> MGSSHHHHHHSQDPNSMTTLTRQDLNFGQVVADVLCEFLEVAVHLILYVREVYPVGIFQKRKKYNVPVQMSCHPELNQYIQDTLHCVKPLLEKNDVEKVVVVILDKEHRPVEKFVFEITQPPLLSISSDSLLSHVEQLLAAFILKISVCDAVLDHNPPGCTFTVLVHTREAATRNMEKIQVIKDFPWILADEQDVHMHDPRLIPLKTMTSDILKMQLYVEERAHKGS;> GNLAGAVEFNDVKTLLREWITTISDPMEEDILQVVKYCTDLIEEKDLEKLDLVIKYMKRLMQQSVESVWNMAFDFILDNVQVVLQQTYGSTLKVT;> MLTPTPDSSPRSTSSPSQSKNGSFTPRTANIL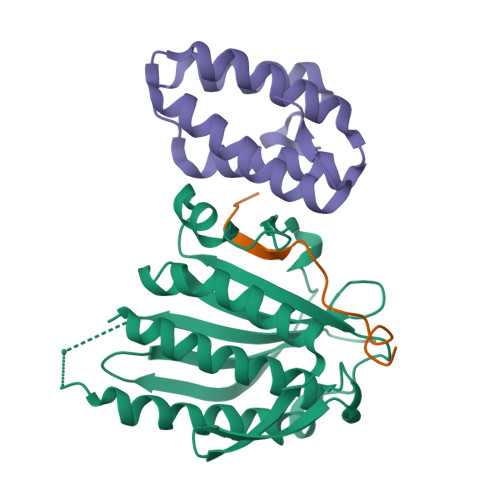KPLMSPPSREEIMATLLDHD> KELNDLEKKYNAHIGVYALDTKSGKEVKFNSDKRFAYAATSKAINSAILLEQVPYNKLNKKVHINKDDIVAYSPILEKYVGKDITLKALIEASMTYSDNTANNKIIKEIGGIKKVKQRLKELGDKVTNPVRYEIELNYYSPKSKKDTSTPAAFGK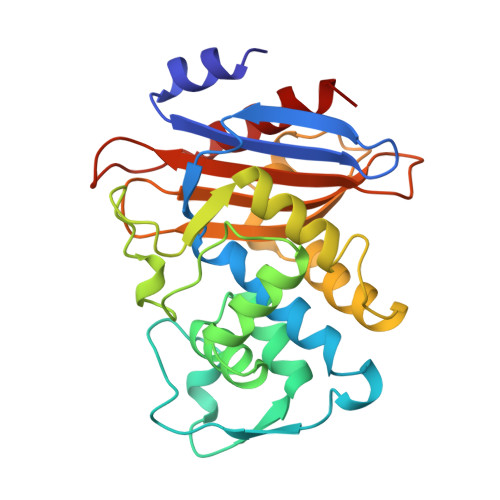TLNKLIANGKLSKENKKFLLDLMLNNKSGDTLIKDGVPKDYKVADKSGQAITYASRNDVAFVYPKGQSEPIVLVIFTNKDNKSDKPNDKLISETAKSVMKEF> GMAEGNTLISVDYEIFGKVQGVFFRKHTQAEGKKLGLVGWVQNTDRGTVQGQLQGPISKVRHMQEWLETRGSPKSHIDKANFNNEKLIEELDYSDF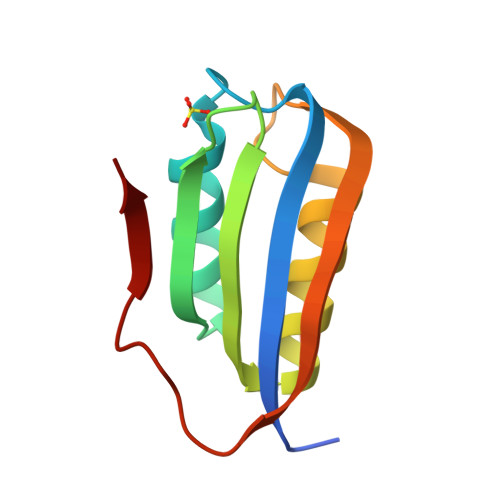QIVA>MVNAEEQQYLNLVQYIINHGEDRPDRTGTGTLSVFAPSPLKFSLRNKTFPLLTTKRVFIRGVIEELLWFIRGETDSLKLREKNIHIWDANGSREYLDSIGLTKRQE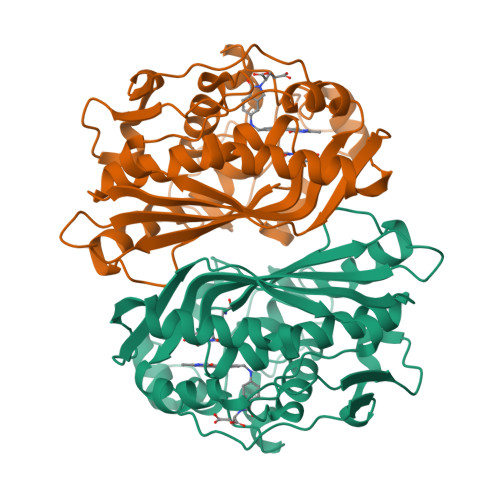GDLGPIYGFQWRHFGAEYIDCKTNYIGQGVDQLANIIQKIRTSPYDRRLILSAWNPADLEKMALPPCHMFCQFYVHIPSNNHRPELSCQLYQRSCDMGLGVPFNIASYALLTCMIAHVCDLDPGDFIHVMGDCHIYKDHIEALQQQLTRSPRPFPTLSLNRSITDIEDFTLDDFNIQNYHPYETIKMKMSI[4x]>GSASLPAELINQIGNRCHPKLYDEGDPSEKLELVTGTNVYITRAQLMNCHVSA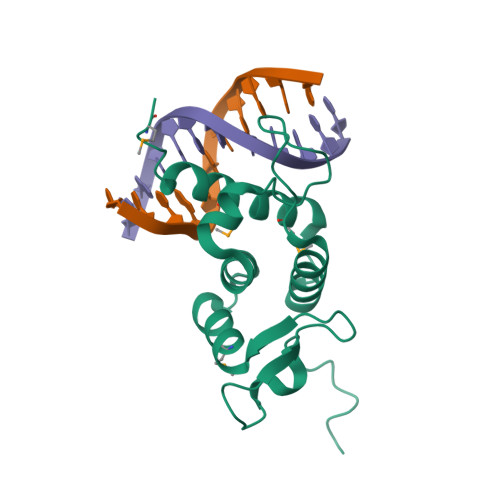GTRHKVLLRRLLASFFDRNTLANSCGTGIRSSTNDPRRKPLDSRVLHAVKYYCQNFAPNFKESEMNAIAADMCTNARRVVRKSWMP[4x]> SNAMNFFTSPFSGIPLDQQVTNPNIIVGKHSYYSGYYHGHSFDDCVRYLHPERDDVDKLVIGSFCSIGSGAVFMMAGNQGHRSDWISTFPFFYQDNDNFADARDGFTRSGDTIIGHDVWIGTEAMIMPGVKIGHGAIIASRSVVTKDVAPYEVVGSNPAKHIKFRFSDVEIAMLLEMAWWNW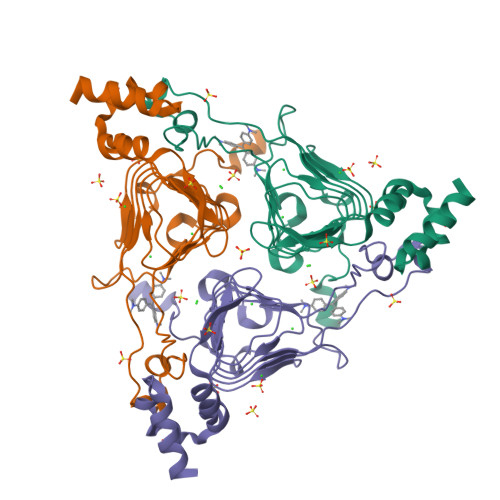PESWLKESMQSLCSSDIEGLYLNWQSKART>[2x]M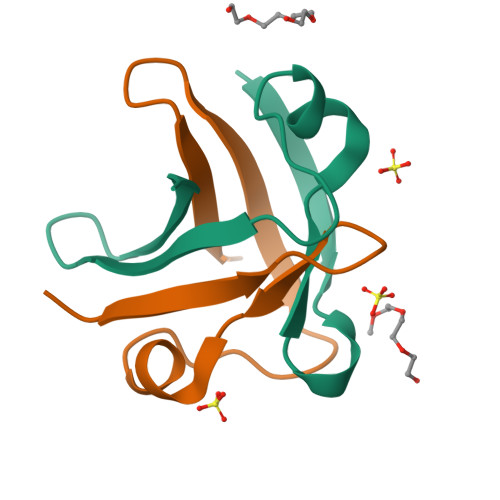AVEEIVKVSRNYQVTIPAKVRQKFQIKEGDLVKVTFDESEGVVKIQLLKEPWK>[2x]CATGTRQSPINIQWKDSVYDPQLAPLRVSYDAASCRYLWNTGYFFQVEFDDSCEDSGISGGPLGNHYRLKQFHFHWGATDEWGSEHAV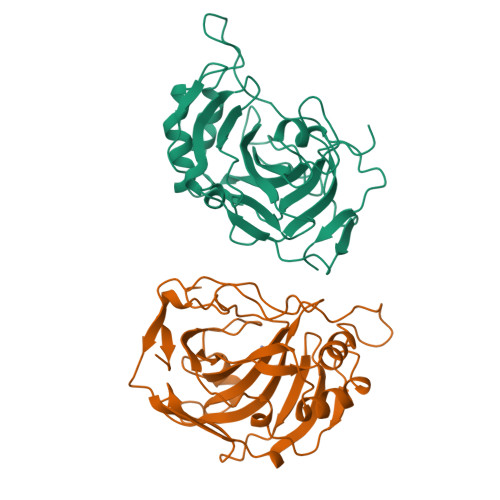DGHTYPAELHLVHWNSTKYENYKKASVGENGLAVIGVFLKLGAHHQALQKLVDVLPEVRHKDTQVAMGPFDPSCLMPACRDYWTYPGSLTTPPLAESVTWIVQKTPVEVSPSQLSMFRTLLFSGRGEEEDVMVNNYRPLQPLRDRKLRSSFRLDRTKMRS>[2x]EETIPLQTLRCYNDYTSHITCRWADTQDAQRLVNVTLIRRVNEDLLEPVSCDLSDDMPWSACPHPRCVPRRCVIPCQSFVVTDVDYFSFQPDRPLGT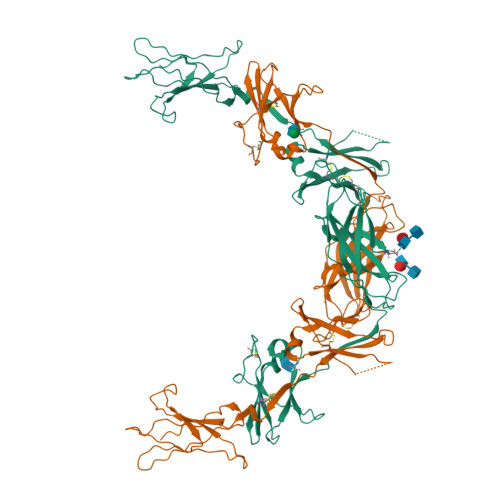RLTVTLTQHVQPPEPRDLQISTDQDHFLLTWSVALGSPQSHWLSPGDLEFEVVYKRLQDSWEDAAILLSNTSQATLGPEHLMPSSTYVARVRTRLAPGSRLSGRPSKWSPEVCWDSQPGDEAQPQNLECFFDGAAVLSCSWEVRKEVASSVSFGLFYKPSPDAGSAVLLREEECSPVLREGLGSLHTRHHCQIPVPDPATHGQYIVSVQPRRAEKHIKSSVNIQMAPPSLQVTKDGDSYSLRWETMKMRYEHIDHTFEIQYRKDTATWKDSKTETLQNAHSMALPALEPSTRYWARVRVRTSRTGYNGIWSEWSEARSWDTE> GMGLGYGSWEIDPKDLTFLKELGTGQFGVVKYGKWRGQYDVAIKMIKEGSMSEDEFIEEAKVMMNLSHEKLVQLYGVCTKQRPIFIITEYMANGSLLNYLREMRHRFQTQQLLEMCKDVCEAMEYLESKQFLHRDLAARNCLVNDQGVVKVSDFGLSRYVLDD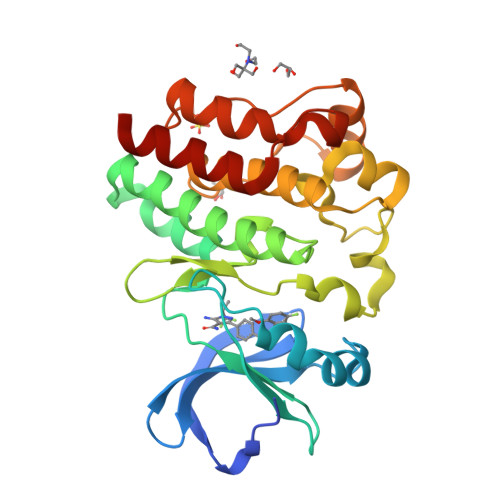EYTSSVGSKFPVRWSPPEVLMYSKFSSKSDIWAFGVLMWEIYSLGKMPYERFTNSETAEHIAQGLRLYRPHLASEKVYTIMYSCWHEKADERPTFKILLSNILDVMDEES> GRISMTVKKLYFIPAGRCMLDHSSVN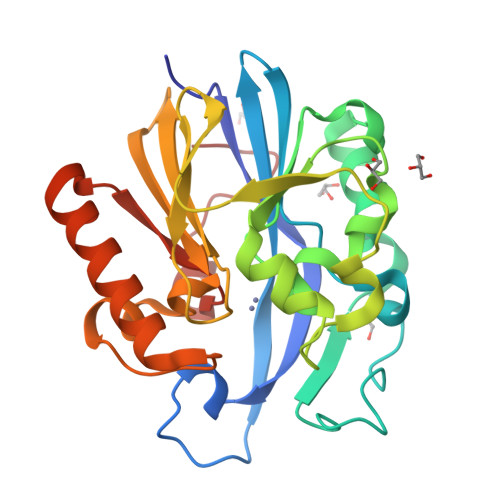SALTPGKLLNLPVWCYLLETEEGPILVDTGMPESAVNNEGLFNGTFVEGQILPKMTEEDRIVNILKRVGYEPDDLLYIISSHLHWDHAGGNGAFTNTPIIVQRTEYEAALHREEYMKECILPHLNYKIIEGDYEVVPGVQLLYTPGHSPGHQSLFIETEQSGSVLLTIDASYTKENFEDEVPFAGFDPELALSSIKRLKEVVKKEKPIIFFGHDIEQEKSCRVFPEYI>VIGRLRGIILEKQPPIVLLETGGVGYEVHMPMTCFYELPEAGQEAIVFTHFVVREDAQLLYGFNNKQERTLFKELIKTNGVGPKLALAILSGMSAQQFVNAVEREELGALVKLPGIGKKTAERLIVEMKDRFK[8x]

The central and universal element in genetic recombination as well as in double strand break repair and in the process of replication fork rescue is a four-way DNA heteroduplex called the Holliday junction. In prokaryotes, the two proteins RuvA and RuvB play critical roles in the processing of the Holliday junction by promoting the ATP-dependent unidirectional strand-exchange reaction known as active branch migration. In bacteria, the Holliday junction is processed by two homo-hexameric AAA+ ATPase RuvB motors, which assemble together with the RuvA–Holliday junction complex to energize the strand-exchange reaction. Here, using time-resolved cryo-electron microscopy, we obtained structures of the ATP-hydrolysing RuvAB complex in seven distinct conformational states, captured during assembly and processing of a Holliday junction. We show that RuvB motors rotate together with the DNA substrate, which, together with a progressing nucleotide cycle, forms the mechanistic basis for DNA recombination by continuous branch migration.

The cryo-EM structure of the RuvAB–HJ complex resolved to a resolution of 8 Å revealed highly flexible and linearly arranged tripartite assemblies, with eight RuvA molecules symmetrically arranged in two tetramers (3.3 Å resolution) and the four-way Holliday junction flanked by, and flexibly connected to,﻿ one or two RuvB hexamers (2.9–4.1 Å resolution) as well as bipartite particles (3.9 Å resolution). In both particle types, DNA enters and exits the RuvA core as a double helix, with one or two hexameric RuvB motors engaging the minor groove of the rejoined DNA. The RuvA core is physically connected to both RuvB motors through RuvAD3. On either side, two RuvAD3 domains are bound to adjacently positioned RuvB subunits, indicating that these domains could cooperate to control the two RuvB AAA+ motors. Notably, all four RuvB-coordinating RuvAD3 domains localize to the same side of the Holliday junction crossover, implying that a single RuvA tetramer might be sufficient to operate both RuvB motors simultaneously. As the DNA substrate already refolds into a double helix within the confinement of the double-tetrameric RuvA core, we propose that the RuvB motor rotation is powered by the rewinding of the translocating DNA. In this view of the RuvAB machinery, the double RuvA tetramer serves an important function in stabilizing the Holliday junction, ensuring that the two DNA substrates can rewind into a double helix and providing a rationale for the rotation of RuvB motors.>[2x]GPGNNELSPVALRQMSCAAGTTQTACTDDNALAYYNTTKGGRFVLALLSDLQDLKWA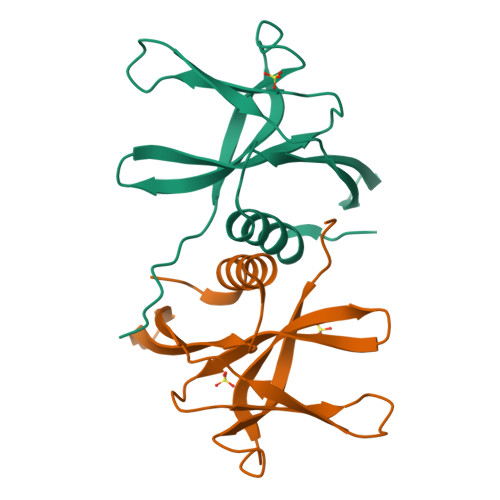RFPKSDGTGTIYTELEPPCRFVTDTPKGPKVKYLYFIKGLNNLNRGMVLGSLAATVRLQ> RRTLWTTPDTSPNCKMSTEKDSKLTLTLTKCGSQVLGNVSLLAVTGEYHQMTATTKKDVKISLLFDENGILLPSSSLSKDYWNYRSDDSIVSQKYNNAVPFMPNLTAYPKPSAQNAKNYSRTKIISNVYLGALTYQPVIITIAFNQETENGCAYSITFTFTWQKDYSAQQFDVTSFTFSYLTQ

Adenoviruses are clinically important, both as human pathogens and as platforms for therapeutic applications. Species D adenovirus type 26 (HAdV-D26) is both a cause of EKC and other diseases and a promising vaccine vector. Here, we demonstrate that HAdV-D26 uses sialic acid–bearing glycans as a primary entry receptor and that this interaction can form a productive infection. We solve the structure of HAdV-D26K in complex with sialic acid [N-acetylneuraminic acid (Neu5Ac)], revealing a similar topology to the known sialic acid–interacting HAdV-D37 fiber knob in the sialic acid–binding pocket, but highlight crucial mechanistic differences likely to enhance HAdV-D26 affinity for sialic acid compared to other types.

Ile324, which is seen to be involved in hydrophobic interactions with the N-acetyl methyl group, can also have multiple conformations. We suggest that the long arm of Ile324 adopts the sialic acid–binding conformation in response to the hydrophobic pressure exerted by sialic acid entering the pocket, minimizing the exposed hydrophobic surface when unbound, holding the methyl group between the short arm of Ile310 and the Tyr312 ring, making this an example of induced fit. We suggest that Gln348 may be labile until the binding of sialic acid.6-METHYL-1,3,5-TRIAZINE-2,4-DIAMINE | C4 H7 N5 | 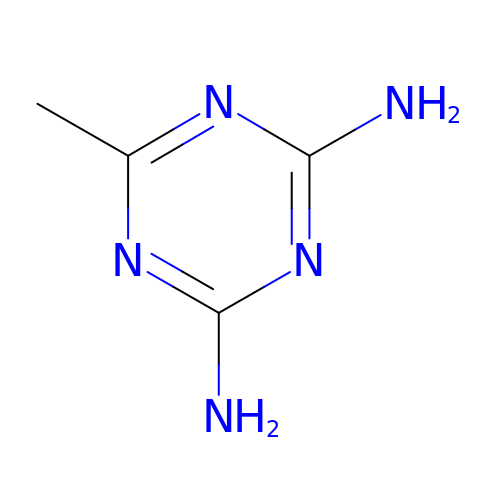NJYZCEFQAIUHSD-UHFFFAOYSA-N>GSKPFTVPILTVEEMTNSRFPIPLEKLFTGPS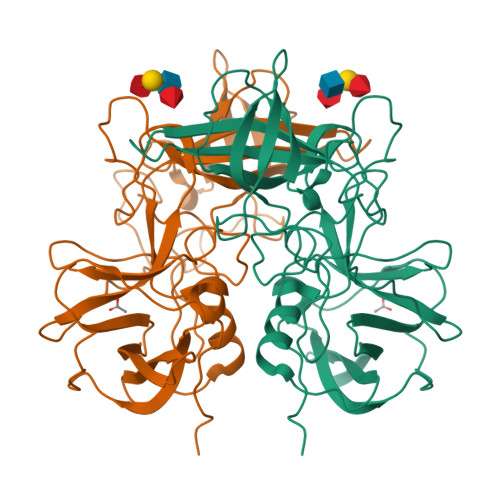GAFVVQPQNGRCTTDGVLLGTTQLSPVNICTFRGDVTHIAGSRNYTMNLASLNWNNYDPTEEIPAPLGTPDFVGKIQGLLTQTTKGDGSTRGHKATVYTGSAPFTPKLGSVQFSTDTENDFETHQNTKFTPVGVIQDGSTTHRNEPQQWVLPSYSGRNVHNVHLAPAVAPTFPGEQLLFFRSTMPGCSGYPNMDLDCLLPQEWVQHFYQEAAPAQSDVALLRFVNPDTGRVLFECKLHKSGYVTVAHTGQHDLVIPPNGYFRFDSWVNQFYTLAPM[2x]> VPFFVNRGGLPVDEATWERMWKHVAKIHPDGEKVAQRIRGATDLPKIPIPSVPTFQPSTPVPERLEAVQRYIRELQYNHTGTQFFEIKKSRPLTGLMDLAKEMTKEALPIKCLEAVILGIYLTNSMPTLERFPISFKTYFSGNYFRHIVLGVNFAGRYGALGMSRREDLMYKPPAFRTLS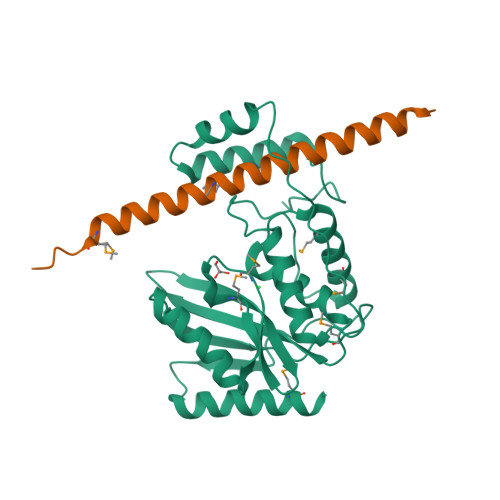ELVLDFEAAYGRCWHVLKKVKLGQSVSHDPHSVEQIEWKHSVLDVERLGRDDFRKELERHARDMRLKI;> RVEKAKQKSAQQELKQRQRAEIYALNRVMTELEQQQFDEFCKQMQPPGE> AGLTRALVARHALGRAEAYDAALLDVAQDHLLYLLS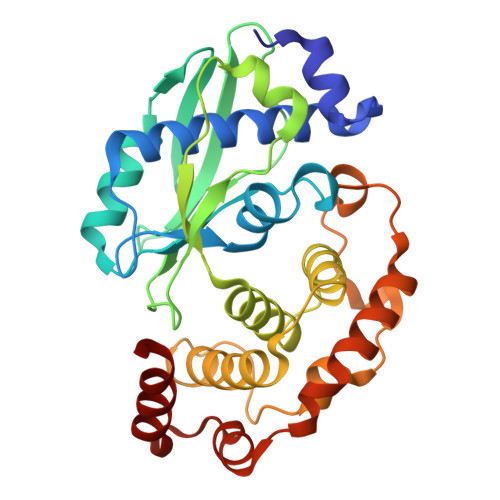QTVQFGDNRLVFKGGTSLRKCRLGNVGRFSTDLDFSAPDDEVVLEVCELIDGARVGGFEFGVQSTRGDGRHWQLRVRHTELGEPRIVASVEFARRPLALPSELLAFIQLPIHKAYGFGLPTLPVVAEAEACAEKLARYRRVALARDLYDLNHFASRTIDEPLVRRLWVLKVWGDVVDDRRGTRPLRVEDVLAARSEHDFQPDSIGVLTRPVAMAAWEARVRKRFAFLTDLDADEQRWAACDERHRREVENALAVLRS>MKKNDFRKNIKLTEPIFNKLKALMKVKDVKQYELIEIILDFYVTNKLSEKEREFFNYQLEELRKEEEEHE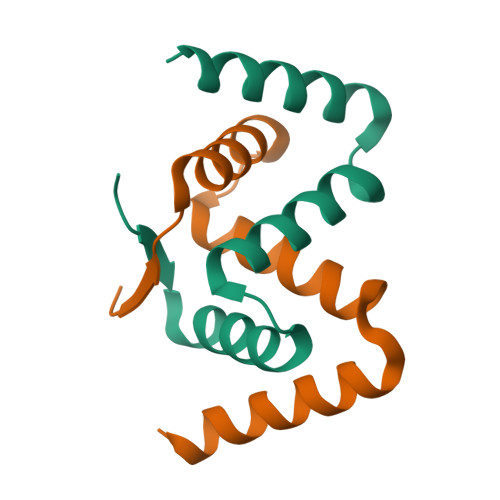[2x]3-[2-(6-AMINO-4-METHYLPYRIDIN-2-YL)ETHYL]-5-{2-[4-METHYL-6-(METHYLAMINO)PYRIDIN-2-YL]ETHYL}BENZONITRILE 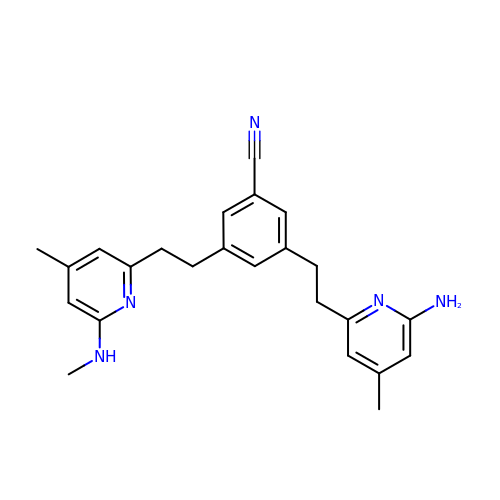| C24 H27 N5 | BRINXWNTHLFLSM-UHFFFAOYSA-N> SMAVKSIKVKLRLDDMPEIRAGLWKLHKEVNAGVRYYTEWLSLLRQENLYRRSPNGDGEQECDKTAEECKAELLERLRARQVENGHRGPAGSDDELLQLARQLYELLVPQAIGAKGDAQQIARKFLSPLADKDAVGGLGIAKAGNKPRWVRMREAGEPGWEEEKEKAETRKSADRTADVLRALADFGLKPLMRVYTDSEMSSVEWKPLRKGQAVRTWDRDMFQQAIERMMSWESWNQRVGQEYAKLVEQKNRFEQKNFVGQEHLVHLVNQLQQDMKEASPGLESKEQTAHYVTGRALRGS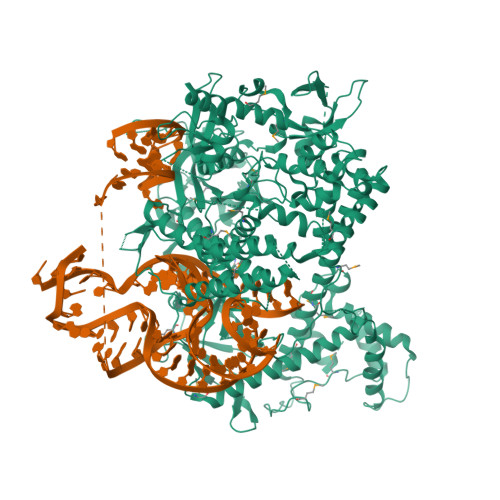DKVFEKWGKLAPDAPFDLYDAEIKNVQRRNTRRFGSHDLFAKLAEPEYQALWREDASFLTRYAVYNSILRKLNHAKMFATFTLPDATAHPIWTRFDKLGGNLHQYTFLFNEFGERRHAIRFHKLLKVENGVAREVDDVTVPISMSEQLDNLLPRDPNEPIALYFRDYGAEQHFTGEFGGAKIQCRRDQLAHMHRRRGARDVYLNVSVRVQSQSEARGERRPPYAAVFRLVGDNHRAFVHFDKLSDYLAEHPDDGKLGSEGLLSGLRVMSVDLGLRTSASISVFRVARKDELKPNSKGRVPFFFPIKGNDNLVAVHERSQLLKLPGETESKDLRAIREERQRTLRQLRTQLAYLRLLVRCGSEDVGRRERSWAKLIEQPVDAANHMTPDWREAFENELQKLKSLHGICSDKEWMDAVYESVRRVWRHMGKQVRDWRKDVRSGERPKIRGYAKDVVGGNSIEQIEYLERQYKFLKSWSFFGKVSGQVIRAEKGSRFAITLREHIDHAKEDRLKKLADRIIMEALGYVYALDERGKGKWVAKYPPCQLILLAELSEYQFNNDRPPSENNQLMQWSHRGVFQELINQAQVHDLLVGTMYAAFSSRFDARTGAPGIRCRRVPARCTQEHNPEPFPWWLNKFVVEHTLDACPLRADDLIPTGEGEIFVSPFSAEEGDFHQIHADLNAAQNLQQRLWSDFDISQIRLRCDWGEVDGELVLIPRLTGKRTADSYSNKVFYTNTGVTYYERERGKKRRKVFAQEKLSEEEAELLVEADEAREKSVVLMRDPSGIINRGNWTRQKEFWSMVNQRIEGYLVKQIRSRVPLQDSACENTGDI>MKITDLELHAVGIPRHTGFVNKHVIVKIHTDEGLTGIGEMSDFSHLPLYSVDLHDLKQGLLSILLGQNPFDLMKINKELTDNFPETMYYYEKGSFIRNGIDNALHDLCAKYLDISVSDFLGGRVKEKIKVCYPIF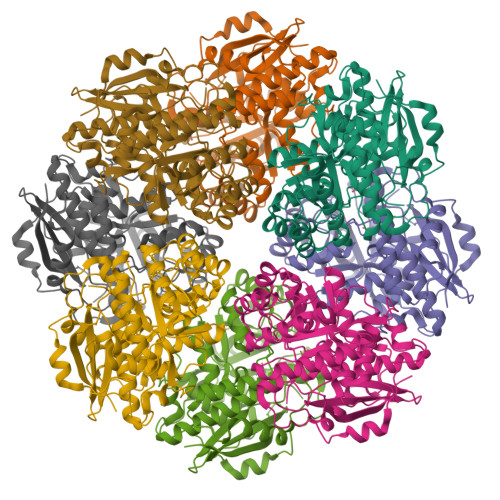RHRFSEEVESNLDVVRQKLEQGFDVFRLYVGKNLDADEEFLSRVKEEFGSRVRIKSYDFSHLLNWKDAHRAIKRLTKYDLGLEMIESPAPRNDFDGLYQLRLKTDYPISEHVWSFKQQQEMIKKDAIDIFNISPVFIGGLTSAKKAAYAAEVASKDVVLGTTQELSVGTAAMAHLGCSLTNINHTSDPTGPELYVGDVVKNRVTYKDGYLYAPDRSVKGLGIELDESLLAKYQVPDLSWDNVTVHQLQDRTADTKS[8x]>[3x]MTCTTGAGVTSGFIDLATYDNLDRALYGGKDATTYFIKEHYPVGWFTKLPTMATRVSGNPA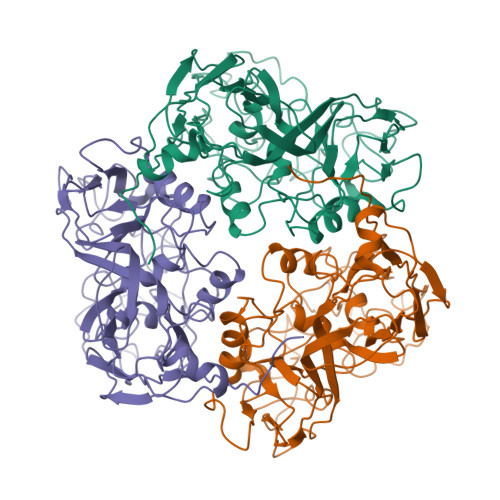FGQEFSVGVPRSGDYVLNAWLTLKTPEIKLLETNRLGANGTVRWTKNLMHNAVEHASLTFNDICAQQFNTAYLDAWTQFNMCEGKRIGYDNMIGNTSDMTNPTPAQGQDGARTLPSKNLVLPLPFFFSRDCGLALPTVVLPYNEIRINIKLRSLQELLVFQNKDTGNVIPISATDIAGGLADTVEAYVYMTVGLVSNVERCAMAGTVRDMVVEQMQAAPTHIVNPQNTNNVHVDMRFSHAVKALFFMVQNVTYKSVGSNYTCVTPVNGPGNTVMEPAMSVDPIKSASLTYENTTRLANMGVEYYSLVQPWYFSASIPVYTGYHMYSYALNVGSVHPSGSTNYGRLTNASITVTMSPESVVAAAGGGNNNSGYNEPQRFALVVIAVNHNVIRIMNGSMGFPIL> WTKEENQSVVVDFLLPTGVYLNFPVSRNANLSTIKQLLWHRAQYEPLFHMLSGPEAYVFTCINQTAEQQELEDEQRRLCDVQPFLPVLRLVAREGDRVKKLINSQISLLIGKGLHEFDSLCDPEVNDFRAKMCQFCEEAAARRQQLGWEAWLQYSFPLQLEPSAQTWGPGTLRLPNRALLVNVKFEGSEESFTFQVSTKDVPLALMACALRKKATVFRQPLVEQPEDYTLQVNGRHEYLYGSYPLCQFQYICSCLHSGLTPHLTMVHSSSILAMRDEQSNPAPQVQKPR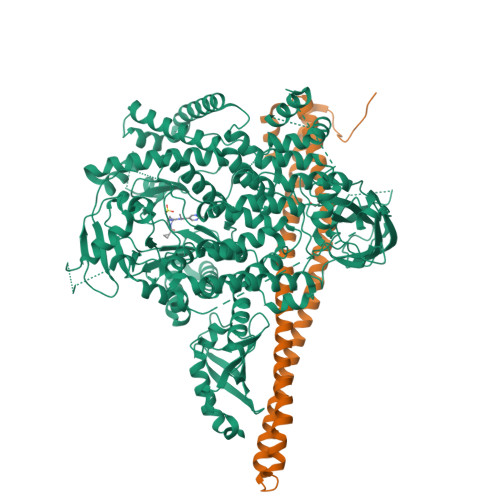AKPPPIPAKKPSSVSLWSLEQPFRIELIQGSKVNADERMKLVVQAGLFHGNEMLCKTVSSSEVSVCSEPVWKQRLEFDINICDLPRMARLCFALYAVIEKAKKARSTKKKSKKADCPIAWANLMLFDYKDQLKTGERCLYMWPSVPDEKGELLNPTGTVRSNPNTDSAAALLICLPEVAPHPVYYPALEKILELGRHSECVHVTEEEQLQLREILERRGSGELYEHEKDLVWKLRHEVQEHFPEALARLLLVTKWNKHEDVAQMLYLLCSWPELPVLSALELLDFSFPDCHVGSFAIKSLRKLTDDELFQYLLQLVQVLKYESYLDCELTKFLLDRALANRKIGHFLFWHLRSEMHVPSVALRFGLILEAYCRGSTHHMKVLMKQGEALSKLKALNDFVKLSSQKTPKPQTKELMHLCMRQEAYLEALSHLQSPLDPSTLLAEVCVEQCTFMDSKMKPLWIMYSNEEAGSGGSVGIIFKNGDDLRQDMLTLQMIQLMDVLWKQEGLDLRMTPYGCLPTGDRTGLIEVVLRSDTIANIQLNKSNMAATAAFNKDALLNWLKSKNPGEALDRAIEEFTLSCAGYCVATYVLGIGDRHSDNIMIRESGQLFHIDFGHFLGNFKTKFGINRERVPFILTYDFVHVIQQGKTNNSEKFERFRGYCERAYTILRRHGLLFLHLFALMRAAGLPELSCSKDIQYLKDSLALGKTEEEALKHFRVKFNEALRESWKTKV;> YQQDQVVKEDNIEAVGKKLHEYNTQFQEKSREYDRLYEDYTRTSQEIQMKRTAIEAFNETIKIFEEQCQTQERYSKEYIEKFKREGNETEIQRIMHNYEKLKSRISEIVDSRRRLEEDLKKQAAEYREIDKRMNSIKPDLIQLRKTRDQYLMWLTQKGVRQKKLNEWLG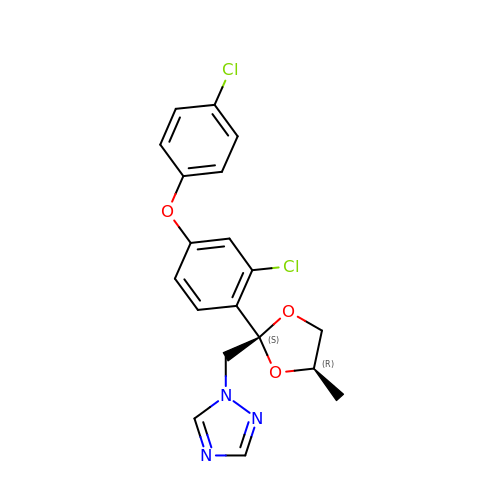1-[[(2~{S},4~{R})-2-[2-chloranyl-4-(4-chloranylphenoxy)phenyl]-4-methyl-1,3-dioxolan-2-yl]methyl]-1,2,4-triazole | C19 H17 Cl2 N3 O3 | BQYJATMQXGBDHF-BFUOFWGJSA-N> MVAPLSVQGNKILANGQPASFSGMSLFWSNTEWGGEKYYNAQVVSWLKSDWNAKLVRAAMGVEDEGGYLTDPANKDRVTQVVDAAIANDMYVIIDWHSHNAHQYQSQAIAFFQEMARKYGANNHVIYEIYNEPLQVSWSNTIKPYAQAVIAAIRAIDPDNLIIVGTPTWSQDVDVAANDPITGYQNIAYTLHFYAGTHGQYLRDKAQTALNRGIALFVTEWGSVNANGDGAVANSETNAWVSFMKTNHISNANWALNDKVEGASALVPGASANGGWVNSQLTASGALAKSIISGWPSYLEHHHHHH

Cellvibrio japonicus is a saprotrophic bacterium which possesses the remarkable ability to grow in isolation using a variety of hemicellulosic polysaccharides as sole carbon sources. It produces a diverse collection of GHs, assembling enzyme systems that can degrade cellulose, xylans, mannans, and xyloglucans, among others. Effective xyloglucan-degrading GH systems (recently reviewed by Attia and Brumer) contain exo-acting glycosidases acting as debranching accessory enzymes and endo-acting enzymes (xyloglucanases) that generate short, branched β-(1,4)-glucan oligomers (xyloglucan oligosaccharides).18−23Exo-acting enzymes are expected to address each of the glycosidic linkages reported in xyloglucan branches, though the reported enzyme diversity falls short of reported branch diversity. The work presented here comprises the design and validation of trisaccharidic xyloglucan (“XyG”)-type cyclophellitol probes and their validation as bona fide, predictive tools for the identification of xyloglucanase activities and their discrimination from cellulase activities within a xyloglucan-elicited C. japonicus degradome.

To determine the molecular basis for the reactivity of ABP-XyG-Cy5 with CjCel5B but not CjCel5C, we crystallized both enzymes and solved their structures by molecular replacement in both unliganded and ABP-bound forms. In contrast, CjCel5B recognizes ABP-XyG-N3 with (−83°, 133°) torsion angles. The consequent twist in the glucose backbone positions the α-(1,6)-xylose residue above W28 and W33, forming a hydrogen bond between O4 and D64. Notably, the active site cleft of CjCel5B is significantly more open beyond the −2 subsite, so we hypothesized that cellulase-specificity in Cel5B is dictated primarily by an inability to accommodate α-(1,6)-xylose residues in the positive subsites. Cel5B showed a ∼14-fold preference for 4MU-GGGG over 4MU-XXXG, roughly in line with its sevenfold preference for ABP-Cel-N3 over ABP-XyG-N3 but highly divergent from its 3000-fold specificity toward carboxymethyl cellulose (CMC) over xyloglucan, supporting our hypothesis. Measurements of irreversible inhibition kinetics showed strong selectivity of Cel5C for ABP-Cel-N3 over ABP-XyG-N3 and only weak selectivity of Cel5B for ABP-Cel-N3 over ABP-XyG-N3, matching in-gel fluorescence results. Pulldowns from saturation cultures using ABP-βGlc-Bio, ABP-Cel-Bio, and ABP-XyG-Bio unambiguously identified Cel5D as the only exclusively ABP-XyG-Bio-reactive band, Cel5C as the exclusively ABP-Cel-Bio-reactive band, and Cel3A, Cel3B, and Cel3D as the ABP-βGlc-reactive bands. The secreted ABP-Cel- and ABP-XyG-reactive band in the arabinoxylan secretome (the intense band in Figure 3A, last lane) was identified as Cel5B. The band of interest was found exclusively in the secretome while Cel5D was found in the cell fraction, so the secretome was collected and concentrated 50-fold by ultrafiltration prior to pulldown using ABP-XyG-Bio.Reversible protein O-GlcNAcylation is achieved by the action of two enzymes, O-GlcNAc transferase (OGT) and O-GlcNAcase (OGA). Although it is unclear whether CpOGA is a physiological OGA, it shows significant in vitro O-GlcNAcase activity on O-GlcNAc proteins in lysates from human cell lines and possesses a putative substrate-binding groove conserved with hOGA (Rao et al., 2006; Schimpl et al., 2010). We report the molecular details of the interaction of a bacterial O-GlcNAcase homolog with three different synthetic glycopeptides derived from characterized O-GlcNAc sites in the human proteome. In addition to extensive contacts with the sugar, O-GlcNAcase recognizes the peptide backbone through hydrophobic interactions and intramolecular hydrogen bonds, while avoiding interactions with the glycopeptide side chains.

To investigate the molecular basis of this substrate specificity, we exploited the catalytic acid mutant of CpOGA, D298N, which is inactive yet unaffected in its ability to bind substrate (Rao et al., 2006). We generated an alternative CpOGA crystal form with a highly accessible active site and determined the structures of CpOGA D298N in complex with the p53-, TAB1-, and hOGA-derived O-GlcNAc peptides. Strikingly, the backbones of all three glycopeptides run in the same direction, together defining the −4 through +3 subsites, and adopt similar conformations near the O-GlcNAc site (maximum Cα shift of 1.8 Å for the −2 to +1 subsites). Notably, all side chains point away from the surface of the enzyme (apart from Trp146 in the p53 peptide, which appears to stack with Asn298 of CpOGA D298N), explaining how a single OGA enzyme is able to recognize >1,000 O-GlcNAc proteins. All three glycopeptides adopt a “V-shaped” conformation that allows the sugar to penetrate the OGA active site. Interestingly, for two of the peptides, this conformation appears to be stabilized by intramolecular hydrogen bonds. For the p53-derived glycopeptide, a hydrogen bond is observed between the aspartic acid in the −1 subsite and the threonine in the +1 subsite. Such intramolecular interactions may stabilize the OGA-bound conformation of these glycopeptides, explaining the significantly lower Kms compared to the TAB1-derived peptide. A notable exception is the tumor suppressor protein p53, where the reported Ser149 O-GlcNAc site resides in a loop that is fully defined in the crystal structure of the p53 DNA binding domain (Cho et al., 1994). Comparing the structure of this loop in the p53 DNA binding domain structure with the glycosylated form reported here, it is apparent that the overall trajectory of the loop is approximately conserved between the two conformations of the peptide (average Cα shift of 2.2 Å), although a number of side chain flips are observed (in particular Trp146).

> GSVGPKTGEENQVLVPNLNPTPENLEVVGDGFKITSSINLVGEEEADENAVNALREFLTANNIEINSENDPNSTTLIIGEVDDDIPELDEALNGTTAENLKEEGYALVSNDGKIAIEGKDGDGTFYGVQTFKQLVKESNIPEVNITDYPTVSARGIVEGFYGTPWTHQDRLDQIKFYGENKLNTYIYAPKDDPYHREKWREPYPESEMQRMQELINASAENKVDFVFGISPGIDIRFDGDAGEEDFNHLITKAESLYDMGVRSFAIYWDNIQDKSAAKHAQVLNRFNEEFVKAKGDVKPLITVPTEYDTGAMVSNGQPRAYTRIFAETVDPSIEVMWTGPGVVTNEIPLSDAQLISGIYDRNMAVWWNYPVTDYFKGKLALGPMHGLDKGLNQYVDFFTVNPMEHAELSKISIHTAADYSWNMDNYDYDKAWNRAIDMLYGDLAEDMKVFANHSTRMDNKTWAKSGREDAPELRAKMDELWNKLSSKEDASALIEELYGEFARMEEACNNLKANLPEVALEECSRQLDELITLAQGDKASLDMIVAQLNEDTEAYESAKEIAQNKLNTALSSFAVISEKVAQSFIQEALS;> QLWVDSTPPPG>MSTRKAVIGYYFIPTNQINNYTETDTSVVPFPVSNITPAKAKQLTHINFSFLDINSNLECAWDPATNDAKARDVVNRLTALKAHNPSLRIMFSIGGWYYSNDLGVSHANYVNAVKTPASRAKFAQSCVRIMKDYGFDGVDIDWQYPQAAEVDGFIAALQEIRTLLNQQTITDGRQALPYQLTIAGAGGAFFLSRYYSKLAQIVAPLDYINLMTYDLAGPWEKVTNHQAALFGDAAGPTFYNALREANLGWSWEELTRAFPSPFSLTVDAAVQQHLMMEGVPSAKIVMGVPFYGRAFKGVSGGNGGQYSSHSTPGEDPYPSTDYWLVGCEECVRDKDPRIASYRQLEQMLQGNYGYQRLWNDKTKTPYLYHAQNGLFVTYDDAESFKY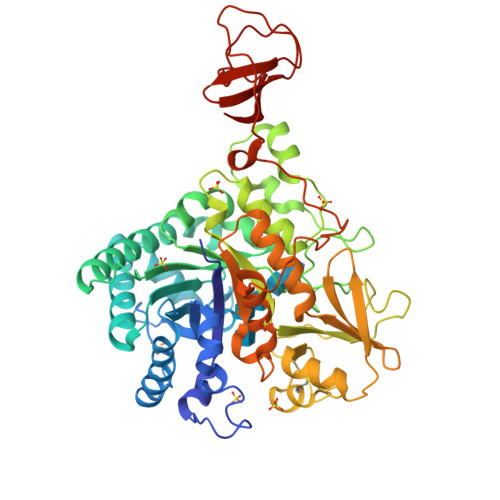KAKYIKQQQLGGVMFWHLGQDNRNGDLLAALDRYFNAADYDDSQLDMGTGLRYTGVGPGNLPIMTAPAYVPGTTYAQGALVSYQGYVWQTKWGYITSAPGSDSAWLKVGRVA[2x]>[10x]MASMIDNRIVKASFRENPVEERKLFPQSSCLMPISVGQAIHEDEKFAAVIKLINASFKQCTILVDDSVQRHTIGIMNHATTEELYQLAVKEGDEWLKRNQRFYKQLTIPFEIMRWDDWYNSPNYINSHLRVQKEYDTNKAFQNAIHANIDDFLTRYLSRFSPADVDHERAFRLCLDYLIEECSVMCLWTEQKYDFEVYPSGRNKAMAATYEFLIKPHHPNYLRPVALRFKKYPAKITGDN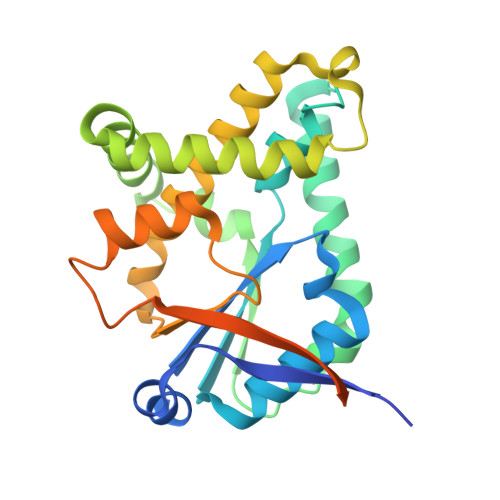LNLIQEQVHENGSMVGGFSRHHHHHH>SNAMAVLEILTAPDPRLRVQSKQVTDVASVQTLIDDLLDTLYATDNGIGLAAPQVGREEAIVVIDLSDNRDQPLVLINPKVVSGSNKEMGQEGCLSVPDYYADVERYTSVVVEALDREGKPLRIETSDFLAIVMQHEIDHLSGNLFIDYLSPLKQQMAMKKVKKHVKNRAR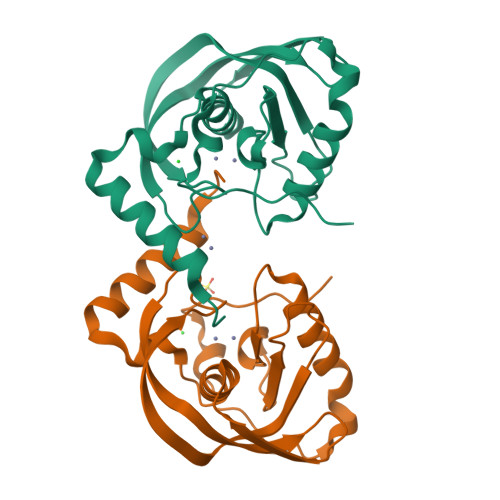[2x]>[2x]MAPITAYSQQTRGLLGCIITSLTGRDK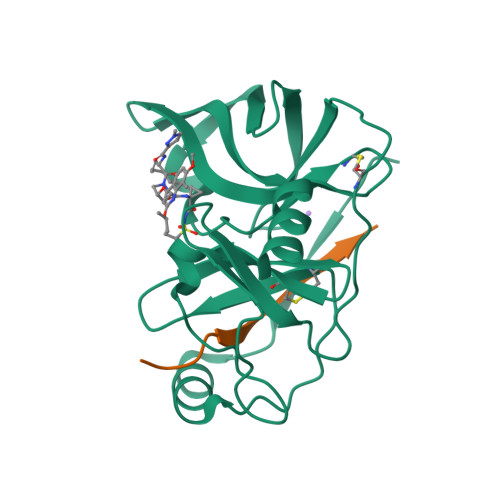NQVDGEVQVLSTATQSFLATCVNGVCWTVYHGAGSKTLAGPKGPITQMYTNVDQDLVGWPAPPGARSMTPCTCGSSDLYLVTRHADVIPVRRRGDSRGSLLSPRPVSYLKGSSGGPLLCPSGHVVGIFRAAVCTRGVAKAVDFIPVESMETTMRASKKKK;>[2x]KKGSVVIVGRIILSGRK>GSHMASPNGQTKPLPALKLALEYIVPAMNKHGICVVDDFLGKETGQQIGDEVRALHDTGKFTDGQLVSQKSDSSKDIRGDKITWIEGKEPGCETIGLLMSSMDDLICHCNGKLGSYKINGRTKAMVACYPGNGTGYVRHVDNCNGDGRCVTCIYYLNKDWDAKVSGGILRIFPE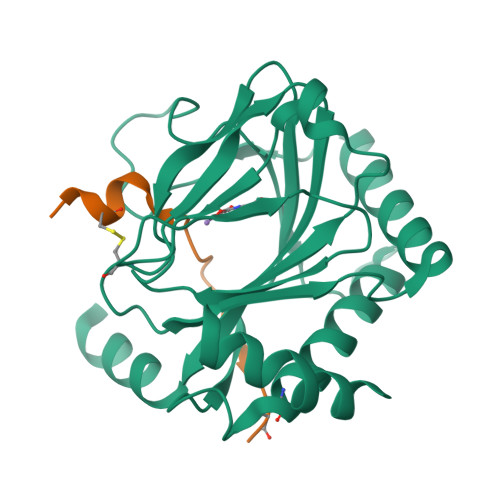GKAQFADIEPKFDRLLFFWSDRRNPHEVQPAYATRYAITVWYFDADERAAAKVKYLTGEKGVRVELNKPSDSVGKDVF[2x];>[2x]DACTLLAPAAGDTIISLCF> ELPQILNDEEISLYSFYDYANKNFNIEKLKQKDDIFSYQKSHIKSSLLVHSDAEQTKVAVEIFSKVLHYMNSNPLVSKKDPADFYSPVKFILTKGLAIESLRDEIYCQLIKQSTSNPIQDLNIRVWELIHF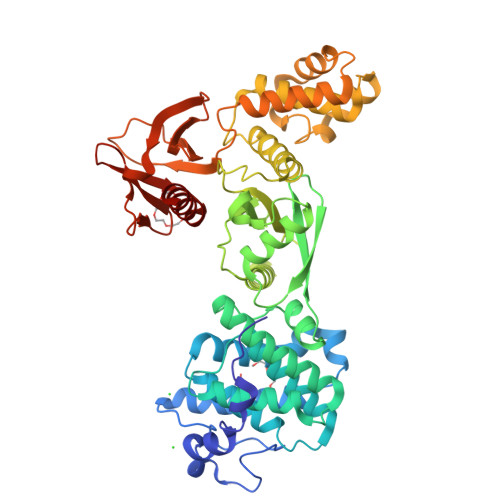TCSTFPPTRKLIKYFAAYLKTTIQQSDVSKSVKDSAQASYFILQRFTLNGARKQVPSVTELESIKENRPIFVRITATDGSLKGLHIDSATTCQESSNDLSQRSRMRVNSKENGFTIIESFNGIERDIAPTDKLCDVLSKVENLQATLSSIQVNFKFVFKKKLFFDNITNNVPTTSINVENEFYYHQLFNDLFNSNYCKDQDYQISIGSLKLQFESSDYTDEIRAWLPGNGRGKYFTTDIEKNRFDDFINKYKSHKGLSPEDAKKQMVQLLEKHPLANCSLVVCEHQSESLPYPKNFVLALNVNGINIYDPATSKMLESVKYSNQSQQNLKSDDKSVSIILENKSTLQAFTGDVQKLVSLIKEYSLYLRN> MADDFGFFSSSESG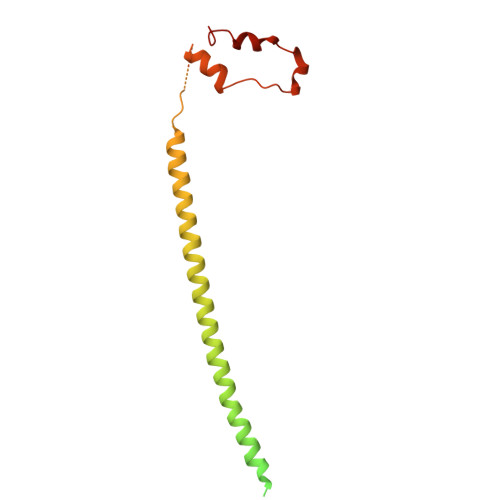APEVAEEDPAAAFLAQQESEIAGIENDEGFGAPAGSQAALAQPGPASGAGPEDMGTTVNGDVFQDANGPADGYAAIAQADRLTQEPESIRKWREEQRKRLQELDAASKVTEQEWREKAKKDLEEWNQRQSEQVEKNKINNRIADKAFYQQPDADIIGYVASEEAFVKESKEETPGTEWEKVAQLCDFNPKSSKQCKDVSRLRSVLMSLKQTPLSR> GPMETTNWIGDENLTGNAEAPAKDDVVPDKNQFRYQKEELAAFCHFGPNTFNEIEWGEHYGNQKPSEIFTLKNDFDAETLVKTLKDAGFKKLIVTAKHHDGFCIWDSEHTEYDVKASGYKNKNGESDILAEISKACTDQNMDMGLYLSPWDIHEPSYGYKDEHGNPTTPDKDAKDYNEFYNNQLEEILGNPKYGNDGHFVEVWMDGA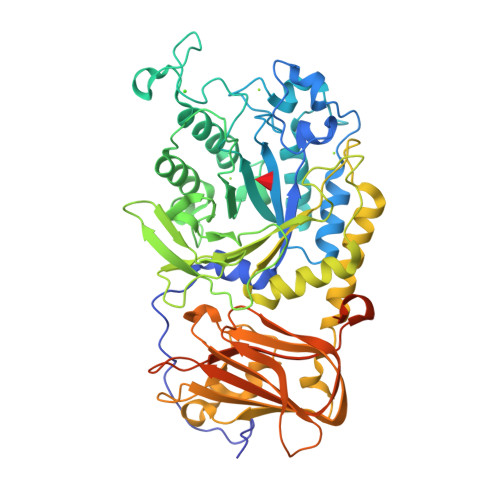KGSGANAQEYDFKKWFKTIQDNEGKAAGYDADCMLFGAEAYTTVRWIGNELGIAGKDTWSKSKVDKDKNTINSNKQGNATVGFEDGDQWTVPEADARITSGWFWGTKKNTPKTMEELSDMYFNSVGHNATLLLNVPPNNQGTVDKAILDRVTEFGNNIKATFKTNLAKAEGASVKVSEVRGGAKEYKPGNMIDDNDETYWATSDGKKSGEILIDLGKETKFDVVSIEEAIQNGQRINNYKVEYRNGDSGTWTLLEEGKTIGAKRLCRTSETTARQIKITVGTCDGKVPMISEIGVYKSTEDMEKPNPIPKGMEVIDVEDKDVADGKGFTFKGKWNPENQPQYING>[2x]GMETTVKIASDSSYAPFEFQNGQKKWVGIDVDIMQEVAKINDWKLEMSYPGFDAALQNLKAGQVDGIIAGMTITDERKETFDFSNPYYTSALTIATTKDSKLSDYSDLKGKAVGAKNGTAAQTWLQENQKKYGYTIKTYSDGVHMFAALSSGNIAGAMDEVPVISYAMKQGQDLAMNFPSISLPGGYGFAVMKGKNSTLVDGFNKALAEMKSNG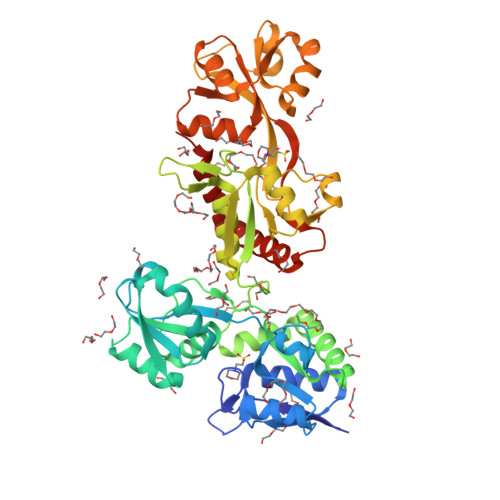DYDKILKKYGITATKKATPKKDVYTIASDNSFAPFEFQNDDKQFTGIDVDLLNAIAKNQGFKLKWNFIGFQAAVDSVQSGHADGMMSGMSITDARKQVFDYGSPYYSSNLTIATSSTDDSIKSWKDLKGKTLGAKNGTASFDYLNAHAKEYGYTVKTFTDATTMYSSLNNGSINALMDDEPVIKYAIKQGQKFATPIKPIPDGQYGFAVKKGSNPELIEMFNNGLANLRANGEYDKIIDKYLESDA>[2x]MKTLMVFDPAMCCSTGVCGTDVDQALVDFSTDVQWL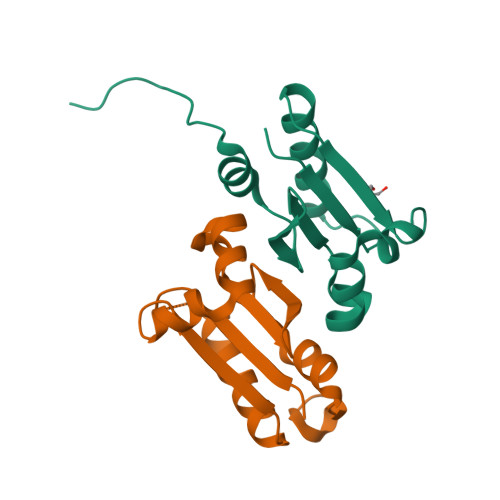KQCGVQIERFNLAQQPMSFVQNEKVKAFIEASGAEGLPLLLLDGETVMAGRYPKRAELARWFGIPLDKVGLAPG> MGHHHHHHSHKIRVAHTPDADDAFMFYAMTHGKVDTWLEIEHVIEDIETLNRKAFNAEYEVTAISAHAYALLDDKYRILSAGASVGDGYGPVVVAKSEISLDGKRIAVPGRYTTANLLLKLAVEDFEPVEMPFDRIIQAVLDEEVDAGLLIHEGQITYADYGLKCVLDLWDW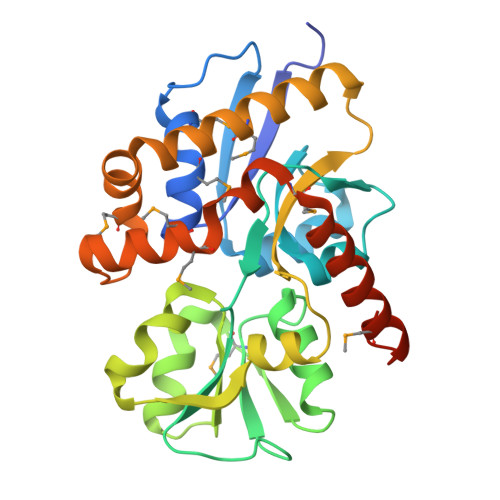WSEQVKLPLPLGLNAIRRDLSVEVQEEFLRAMRESIAFAIENPDEAIEYAMKYSRGLDRERAKRFAMMYVNDYTYNMPESVDAALKKLYEMAEAKGLIKMPKLDILRL>[9x]MEFTVSTTEDLQRYRTECVSSLNIPADYVEKFKKWEFPEDDTTMCYIKCVFNKMQLFDDTEGPLVDNL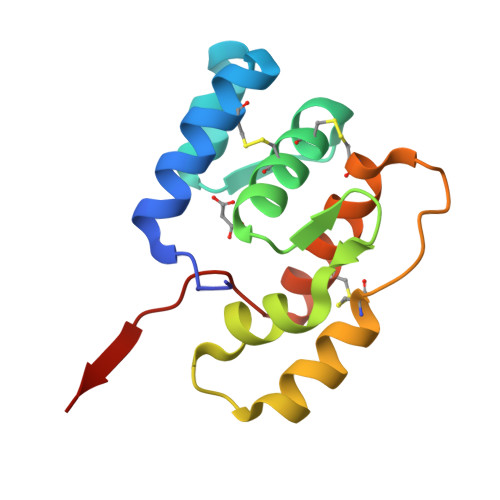VHQLAHGRDAEEVRTEVLKCVDKNTDNNACHWAFRGFKCFQKNNLSLIKASIKKD> MDESLEHQTQTHDQESEIVTEGSAVVHSEPSQEGNVPPK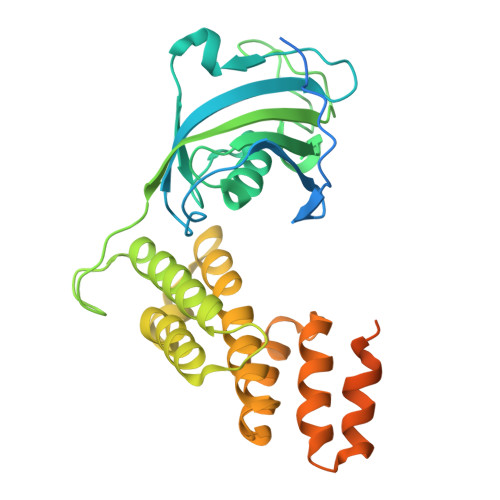VDSEAEVLDEKVSKQIIKEGHGSKPSKYSTCFLHYRAWTKNSQHKFEDTWHEQQPIELVLGKEKKELAGLAIGVASMKSGERALVHVGWELAYGKEGNFSFPNVPPMADLLYEVEVIGFDETKEGKARSDMTVEERIGAADRRKMDGNSLFKEEKLEEAMQQYEMAIAYMGDDFMFQLYGKYQDMALAVKNPCHLNIAACLIKLKRYDEAIGHCNIVLTEEEKNPKALFRRGKAKAELGQMDSARDDFRKAQKYAPDDKAIRRELRALAEQEKALYQKQKEMYKGIFKGKDEGGAKSKS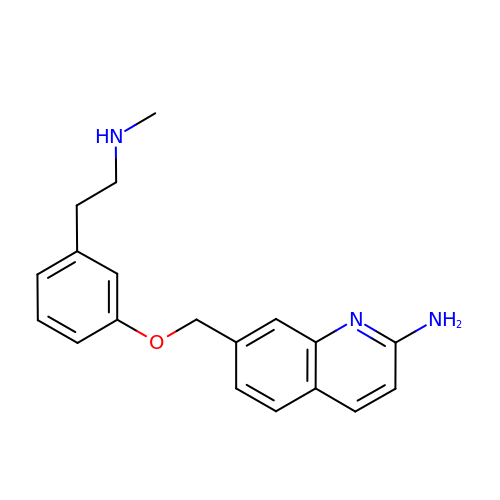7-[[3-[2-(methylamino)ethyl]phenoxy]methyl]quinolin-2-amine | C19 H21 N3 O | IHPWSPZSFKTYCX-UHFFFAOYSA-N>[2x]AEKPKLHYF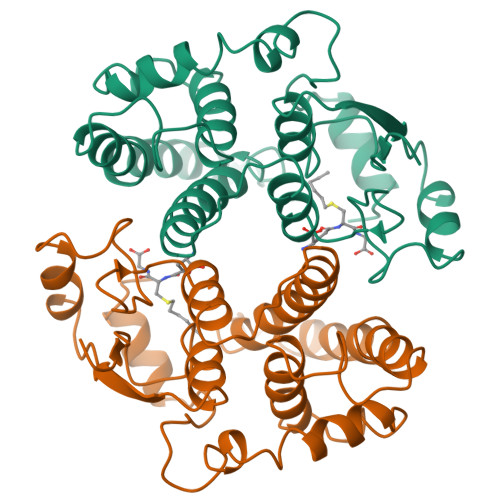NARGRMESTRWLLAAAGVEFEEKFIKSAEDLDKLRNDGYLMFQQVPMVEIDGMKLVQTRAILNYIASKYNLYRKDIKEKALIDMYIEGIADLGEMILLLPFTQPEEQDAKLALIKEKIKNRYFPAFEKVLKSHGQDYLVGNKLSRADIHLVELLYYVEELDSSLISSFPLLKALKTRISNLPTVKKFLQPGSPRKPPMDEKSLEEARKIFRF>[2x]GMGKRGREGTLDKARC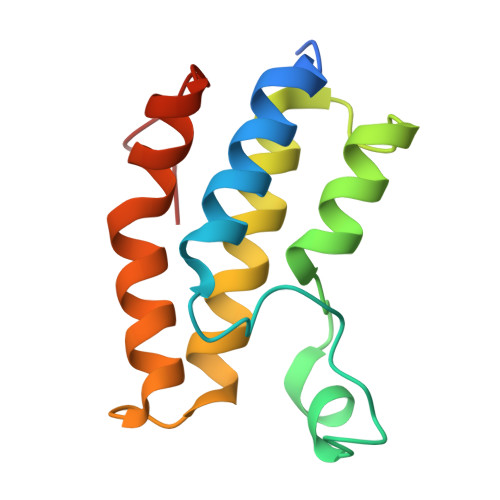LAFVHQLWDKDKLKMFHHPISAAELPDYHKVINYPVDLSTIRQGIESGKYDSDADVQNAVAQMIANALEYNAKGTEWHQQALSFRSIYLDVARQCGLSVDDDAAY Synaptic vesicle glycoprotein 2a (SV2A), a putative membrane transporter in the synaptic vesicles (SVs), has been identified as a target of LEV and BRV. SV2A also serves as a receptor for botulinum neurotoxin (BoNT), which is the most toxic protein and has paradoxically emerged as a potent reagent for therapeutic and cosmetic applications. SV2 family proteins belong to the major facilitator superfamily (MFS) with 12 predicted transmembrane helices. In addition to the transmembrane domain (TMD) core, a cytosolic N-terminal region and a large fourth luminal domain (LD4) are present.

In addition to the monomeric SV2A–HCA2–LEV complex, we also obtained the cryo-EM reconstruction of the dimeric assembly of the SV2A–HCA2–LEV complex to 2.90 Å resolution, in which two SV2A–HCA2–LEV complexes are assembled through the LD4–LD4 interaction, positioning two SV2A TMDs in a near perpendicular configuration. The cryo-EM structure of the dimeric assembly of the SV2A–HCA2–LEV complex is formed through the LD4–LD4 interaction, in which the open edge of the β-strand from each LD4 forms an anti-parallel β-sheet. The TMDs in the dimeric complex are in near perpendicular orientation. The association of LD4 may contribute to accumulating the glycans to form a gel matrix. Further study is necessary to address the structural role of SV2A in SV morphology.

>[2x]MDYKDDDDKEEGFRDRAAFIRGAKDIAKEVKKHAAKKVVKGLDRVQDEYSRRSYSRFEEEDDDDDFPAPSDGYYRGEGTQDEEEGGASSDATEGHDEDDEIYEGEYQGIPRAESGGKGERMADGAPLAGVRGGLSDGEGPPGGRGEAQRRKEREELAQQYEAILRECGHGRFQWTLYFVLGLALMADGVEVFVVGFVLPSAEKDMCLSDSNKGMLGLIVYLGMMVGAFLWGGLADRLGRRQCLLISLSVNSVFAFFSSFVQGYGTFLFCRLLSGVGIGGSIPIVFSYFSEFLAQEKRGEHLSWLCMFWMIGGVYAAAMAWAIIPHYGWSFQMGSAYQFHSWRVFVLVCAFPSVFAIGALTTQPESPRFFLENGKHDEAWMVLKQVHDTNMRAKGHPERVFSVTHIKTIHQEDELIEIQSDTGTWYQRWGVRALSLGGQVWGNFLSCFGPEYRRITLMMMGVWFTMSFSYYGLTVWFPDMIRHLQAVDYASRTKVFPGERVEHVTFNFTLENQIHRGGQYFNDKFIGLRLKSVSFEDSLFEECYFEDVTSSNTFFRNCTFINTVFYNTDLFEYKFVNSRLINSTFLHNKEGCPLDVTGTGEGAYMVYFVSFLGTLAVLPGNIVSALLMDKIGRLRMLAGSSVMSCVSCFFLSFGNSESAMIALLCLFGGVSIASWNALDVLTVELYPSDKRTTAFGFLNALCKLAAVLGISIFTSFVGITKAAPILFASAALALGSSLALKLPETRGQVLQ;>KNIVNTSILSIVYKKDDLIDLSRYGAKINIGDRVYYDSIDKNQIKLINLESSTIEVILKNAIVYNSMYENFSTSFWIKIPKYFSKINLNNEYTIINCIENNSGWKVSLNYGEIIWTLQDNKQNIQRVVFKYSQMVNISDYINRWIFVTITNNRLTKSKIYINGRLIDQKPISNLGNIHASNKIMFKLDGCRDPRRYIMIKYFNLFDKELNEKEIKDLYDSQSNSGILKDFWGNYLQYDKPYYMLNLFDPNKYVDVNNIGIRGYMYLKGPRGSVVTTNIYLNSTLYEGTKFIIKKYASGNEDNIVRNNDRVYINVVVKNKEYRLATNASQAGVEKILSALEIPDVGNLSQVVVMKSKDDQGIRNKCKMNLQDNNGNDIGFIGFHLYDNIAKLVASNWYNRQVGKASRTFGCSWEFIPVDDGWGESSL[2x]>[16x]MKKITLLLAGSALLLSGCAGVKSSFDCDATTSDTCMTMTKANQLARDKAAKQAGKPAAGGLPSLVNLPATSAVEVPSASRSAVTPPSGTRTVSTTPPVSAGTSAGVNTNTTTSTLTPRPVAGTPVTTTPSSVAYRPVVSVVTPTPSCQNVRCDNPGTVHPQRSRDQIATVWIAPWVDSDNAFHQPGRVSFVVSPADWVLPARVN;>MANVNKVVRRRQVALLIALVLGIGAGGAGTWMVSEMNLKKAPPAKAPKGEPAPDMTGVVNQSFDNKVQRSAIAEAQRLNKETQTEIKKLRTEMGLVSRDLKGSQDRIRELEDQ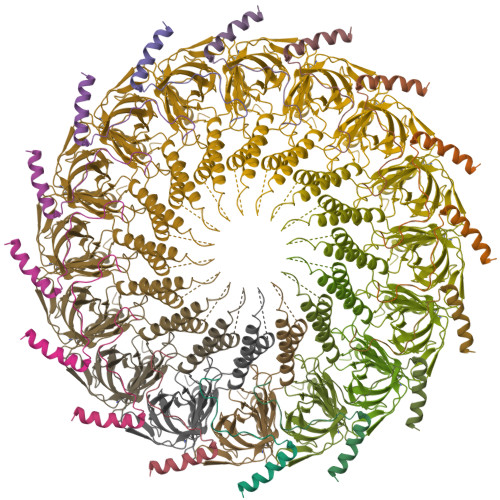NQLLQTQLEAGKNFDSLSAEPLPGALASQGKPAPAGNVPPPTSFWPAGGGQAPAAPVMTPIQRPGMMDSQEFSLPDTGPKKPRFPWISSGSFVEAIVVEGADANASVTGDKNTAPMQLRLTGKVQMPNDEEFDLTGCFVTLEAWGDVSSERAIVRSRSISCKLGDDDIDQKIAGHVSFMGKNGIKGEVVMRNGQILLYAGGAGFLDGIGKGIEKASSTTVGVGATASMSAADIGQAGLGGGVSSAAKTLSDYYIKRAEQYHPVIPIGAGNEVTLVFQDGFQLETLEEARAKAAARKKQNQPSASSTPAAMPGNTPDMLKQLQDFRVGDTVDPATGQVVTQ[16x]>MGSMAASTPVVVDIHTHMYPPSYIAMLEKRQTIPLVRTFPQADEPRLILLSSELAALDAALADPAAKLPGRPLSTHFASLAQKMHFMDTNGIRVSVISLANPWFDFLAPDEAPGIADAVNAEFSDMCAQHVGRLFFFAALPLSAPVDAVKASIERVKNLKYCRGIILGTSGLGKGLDDPHLLPVFEAVADAKLLVFLHPHYGLPNEVYGPRSEEYGHVLPLALGFPMETTIAVARMYMAGVFDHVRNLQMLLAHSGGTLPFLAGRIESCIVHDGHLVKTGKVPKDRRTIWT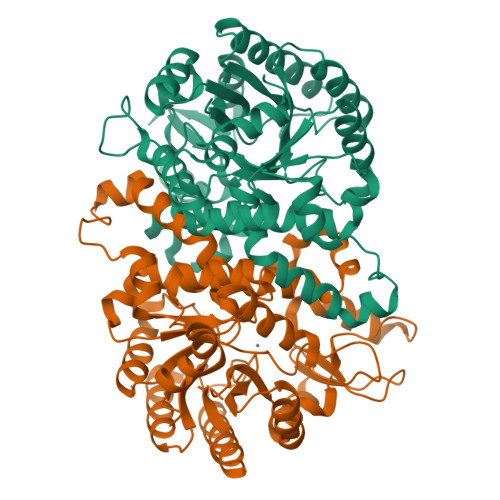VLKEQIYLDAVIYSEVGLQAAIASSGADRLMFGTDHPFFPPIEEDVQGPWDSSRLNAQAVIKAVGEGSSDAAAVMGLNAVRVLSLKAELEHHHHHH[4x]> TKQVSQNITKNTEDILASITKEYATQTQGIFGEMIALNKSISGTLTEMFRSTSKEDLDIDNITNIITNTFDNSAYSNFTYLYLIDPPEYFKEESKFFNTQSGKFVMLYADEEKDNKGGIKAIQASDEIANLQVVQDILKKAKYGENKVYIGRPIKMNLEGQDFDAVNVAIPIFDRKNQVVGVIGMTLDFSDIATYLLDPKGQKYDGELRVLLNSDGFMAIHPNKNLVLKNLKDINPNKGAQETYKAISEGKNGVFNYIASDGDDSYAAINSFKVQ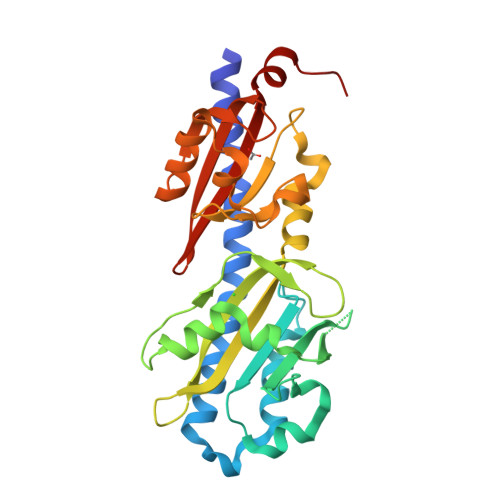DSSWAVLVTAPKYSVFKPLKKL> MTMAANTDRAVLQAALPPLSGSLPIPGLSASVRVRRDAWGIPHIKASGEADAYR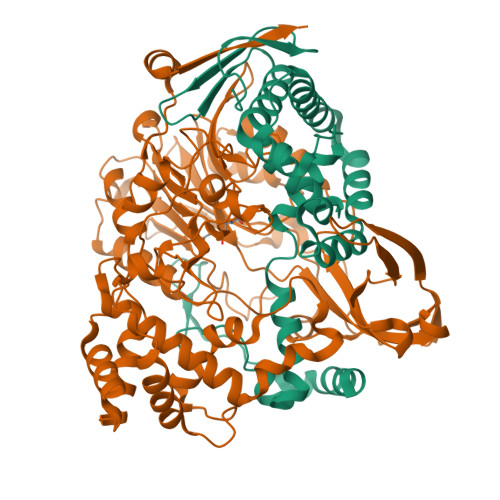ALGFVHSQDRLFQMELTRRKALGRAAEWLGAEAAEADILVRRLGMEKVCRRDFEALGVEAKDMLRAYVAGVNAFLASGAPLPVEYGLLGAEPEPWEPWHSIAVMRRLGLLMGSVWFKLWRMLALPVVGAANALKLRYDDGGRDLLCIPPGAEADRLEADLATLRPAVDALLKAMG;> SNNWAVAPGRTATGRPILAGDPHRVFEIPGFYAQHHLACDRFDMIGLTVPGVPGFPSFAHNGKVAYCVTSAFMDIHDLYLEQFAGEGRTARFGNDFEPVAWSRDRIAVRGGADREFDIVETRHGPVIAGDPRDGAALTLRSVQFAETDLSFDCLTRMPGASTVAQLYDATRGWGLIDHNLVAGDVAGSIGHLVRARVPSRPRENGWLPVPGWSGEHEWRGWIPHEAMPRVIDPPGGIIVTANNRVVADDHPDYLCTDCHPPYRAERIMKRLVANPAFAVDDAAAIHADTLSPHVGLLRRRLEALGARDDSAAEGLRQMLVAWDGRMDAASEVASAYNAFRRALTRLVTDRSGLEQAISHPFAAVAPGVSPQGQVWWAVPTLLRDDDAGMLKGWSWDQALSEALSVASQNLTGRSWGEEHRPRFTHPLATQFPAWAGLLNPASRPIGGDGDTVLANGLVPSAGPQATYGALSRYVFDVGNWDNSRWVVFHGASGHPASAHYADQNAPWSDCAMVPMLYSWDRIAAEAVTSQELVPALEHHHHHH Oligosaccharyltransferase (OST) is the central enzyme of N-linked protein glycosylation. It catalyzes the transfer of a pre-assembled glycan, GlcNAc2Man9Glc3, from a dolichyl-pyrophosphate donor to acceptor sites in secretory proteins in the lumen of the endoplasmic reticulum. In higher metazoans and fungi, OST is a multimeric complex composed of eight subunits spatially arranged in three subcomplexes that are formed during OST assembly. Subcomplex I contains OST1 and OST5; subcomplex II contains OST3 (or OST6), STT3, and OST4; and subcomplex III contains OST2, WBP1, and SWP1.

We performed single-particle cryo-EM analysis of a sample containing nanodisc-reconstituted yeast OST, MnCl2, chemo-enzymatically generated Dol20-PP-GlcNAc2Man9Glc3, and the non-reactive peptide TAMRA-YA(Dab)ATS-NH2, where the acceptor asparagine was replaced by 2,4-diaminobutanoic acid (Dab)31,41–43. The generation of the substrate analogs TAMRA-YA(Dab)ATS and Dol20-PP-GlcNAc2Man9Glc3 enabled us to visualize a ternary complex of eukaryotic OST, and well-defined EM density covering bound peptide, which allowed us to build the complete hexapeptide chain. Intriguingly, clear density was also observed for the attached TAMRA fluorophore in a pocket formed between the subunits STT3 and OST3, a location that would accommodate the nascent polypeptide chain N-terminal to the glycosylation sequon. The side chain of the Dab residue is lodged in this tunnel, with its terminal amino group positioned at a distance of 3.3 Å from the C-1 of the reducing-end GlcNAc of the glycan donor. This suggests that our structure reflects a state preceding the nucleophilic attack on the reducing end GlcNAc, akin to a pseudo-Michaelis complex. In this conformation, two residues from the EL5 contribute and complete the active site of the enzyme: Glu350 and Arg328. The second, Arg328, provides a salt bridge with the pyrophosphate group of bound LLO. This interaction is not present in the binary complex of OST with bound LLO state, where the pyrophosphate group only interacts with Trp208 and Arg404. The manganese (II) ion is coordinated by residues of the DxD/E motif47 (Asp166 and Glu168), the catalytic residues Asp47 and Glu350, and by the pyrophosphate group of the LLO. Upon binding of an acceptor peptide, the complete EL5 and TM9 become ordered, resulting in a catalytically active state.

> MGSDRSCVLSVFQTILKLVIFVAIFGAAISSRLFAVIKFESIIHEFDPWFNYRATKYLVNNSFYKFLNWFDDRTWYPLGRVTGGTLYPGLMTTSAFIWHALRNWLGLPIDIRNVCVLFAPLFSGVTAWATYEFTKEIKDASAGLLAAGFIAIVPGYISRSVAGSYDNEAIAITLLMVTFMFWIKAQKTGSIMHATCAALFYFYMVSAWGGYVFITNLIPLHVFLLILMGRYSSKLYSAYTTWYAIGTVASMQIPFVGFLPIRSNDHMAALGVFGLIQIVAFGDFVKGQISTAKFKVIMMVSLFLILVLGVVGLSALTYMGLIAPWTGRFYSLWDTNYAKIHIPIIASVSEHQPVSWPAFFFDTHFLIWLFPAGVFLLFLDLKDEHVFVIAYSVLCSYFAGVMVRLMLTLTPVICVSAAVALSKIFDIYLDFKTSDRKYAIKPAALLAKLIVSGSFIFYLYLFVFHSTWVTRTAYSSPSVVLPSQTPDGKLALIDDFREAYYWLRMNSDEDSKVAAWWDYGYQIGGMADRTTLVDNNTWNNTHIAIVGKAMASPEEKSYEILKEHDVDYVLVIFGGLIGFGGDDINKFLWMIRISEGIWPEEIKERDFYTAEGEYRVDARASETMRNSLLYKMSYKDFPQLFNGGQATDRVRQQMITPLDVPPLDYFDEVFTSENWMVRIYQLKKDDAQGRTLRDVGELTRSSTKTRRSIKRPELGLRV;> MISDEQLNSLAITFGIVMMTLIVIYHAVDSTMSPKNRTLQVDGGSGGSLEVLFQGPTETSQVAPA;> MTYEQLYKEFHSSKSFQPFIHLDTQPKFAICGLIVTLAVLSSALFAVGSKSSYIKKLFFYTILSVIGSLFAGLTTVFASNSFGVYV;> MAKAPKANTPKVTSTSSAVLTDFQETFKTSKRAYFAQIEKYPKLKLIDTFCFFLVLLGVIQCTFIILIRDNFPFNAFLAGFIICVGQFVLLMSLRLQLCNSFPGISKNRAFAEFIVASLILHFVCLHFIN;> MRQVWFSWIVGLFLCFFNVSSAAQYEPPATWENVDYKRTIDVSNAYISETIEITIKNIASEPATEYFTAFESGIFSKVSFFSAYFTNEATFLNSQLLANSTTAPGDDGESEIRYGIIQFPNAISPQEEVSLVIKSFYNTVGIPYPEHVGMSEEQHLLWETNRLPLSAYDTKKASFTLIGSSSFEEYHPPNDESLLGKANGNSFEFGPWEDIPRFSSNETLAIVYSHNAPLNQVVNLRRDIWLSHWASTIQFEEYYELTNKAAKLSKGFSRLELMKQIQTQNMRQTHFVTVLDMLLPEGATDHYFTDLVGLVSTSHAERDHFFIRPRFPIFGGWNYNFTVGWTNKLSDFLHVSSGSDEKFVASIPILNGPPDTVYDNVELSVFLPEGAEIFDIDSPVPFTNVSIETQKSYFDLNKGHVKLTFSYRNLISQVANGQVLIKYDYPKSSFFKKPLSIACYIFTALMGVFVLKTLNMNVTN;> MQFFKTLAALVSCISFVLAYVAQDVHVSFPSTAGKSRVMIGKVEPRIGIDETVPTTITVEDPNEVIQVNFAIESTNKPFQNTLLIGLPNKNLEMAFEPEIKDNGKLSMYKYRIDLAKLDAALLQEASRSPEPIKATLILASSTAKPKENLFREILQLNLNFDVDHSDSSLVDKFGIKPEIHHIFHAEPKRVAKPIAVIFVLIIFITILSLIVTWLNSCAAAFNNIPTGVTAVYFLGFIATIVGFEVIFARYYLGTSIFETLFSSLYLGAPGLLTSTKFLRSFG;> MRTDWNFFFCILLQAIFVVGTQTSRTLVLYDQSTEPLEEYSVYLKDLEQRNYKLEYLDINSTSTTVDLYDKEQRLFDNIIVFPTKGGKNLARQIPVKQLIKFFENEGNILCMSSPGAVPNTIRLFLNELGIYPSPKGHVIRDYFSPSSEELVVSSNHLLNKYVYNARKSEDFVFGESSAALLENREQIVPILNAPRTSFTESKGKCNSWTSGSQGFLVVGFQNLNNARLVWIGSSDFLKNKNQDSNQEFAKELLKWTFNEKSVIKSVHAVHSHADGTSYDEEPYKIKDKVIYSVGFSEWNGEEWLPHIADDIQFELRQVDPYYRLTLSPSGNDSETQYYTTGEFILPDRHGVFTFLTDYRKIGLSFTTDKDVKAIRHLANDEYPRSWEISNSWVYISAICGVIVAWIFFVVSFVTTSSVGKKLETFKKTN;> MNWLFLVSLVFFCGVSTHPALAMSSNRLLKLANKSPKKIIPLKDSSFENILAPPHENAYIVALFTATAPEIGCSLCLELESEYDTIVASWFDDHPDAKSSNSDTSIFFTKVNLEDPSKTIPKAFQFFQLNNVPRLFIFKPNSPSILDHSVISISTDTGSERMKQIIQAIKQFSQVNDFSLHLPMDWTPIITSTIITFITVLLFKKQSKLMFSIISSRIIWATLSTFFIICMISAYMFNQIRNTQLAGVGPKGEVMYFLPNEFQHQFAIETQVMVLIYGTLAALVVVLVKGIQFLRSHLYPETKKAYFIDAILASFCALFIYVFFAALTTVFTIKSPAYPFPLLRLSAPFK;> YAAATSA> MQCTSRLLGGYMMYHRKSMSTMRYSKWKGARGG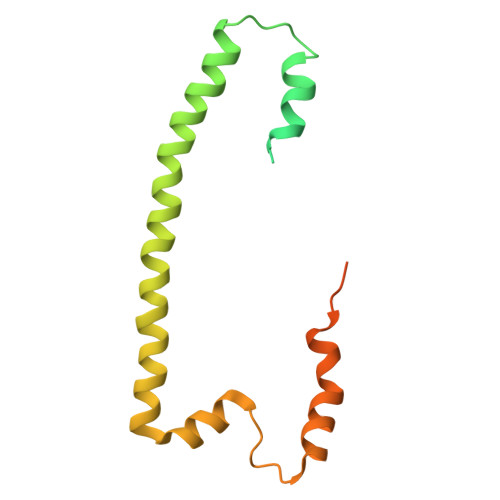LSHFYNRTAMLEKVPVNMPVSIVDRRMMAYVHRSRLRHFQLFRSYQQKSNSTECKLREGEFLRRRWHRQLQKSFIAFMQFKTMKVLEEQAKLVSQYGQASVNAALGDPQAAAGDVAHERKYAALHRRVQTLPRIQLVPKHVATMKQIHNDRFNYRWRVN>[4x]ETGFVNKDQIAKDVKQFYDQALQQAVVDDDANNAKAVVKTFH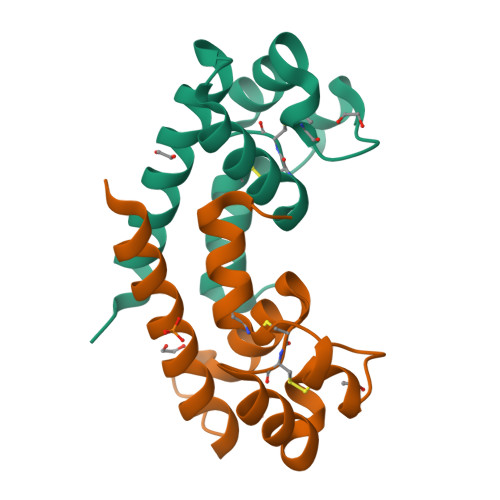ETLDCCGSSTLTALTTSVLKNNLCPSGSNIISNLFKEDCHQKIDDLFSGKGTKHHHHHH> VNFPNIPAEGVRFRLRARDSGYVIYSRTENDPLVWHYNGPPYDDQLFTLIHGTGSRLNLYAIKSVPNGRVLFSRNSASPTVGNIVGDGTYNDNWFQFIQDDNDANSFRIYSLASDSVLYSRTTGAPQFGNYTGPKFDDQLW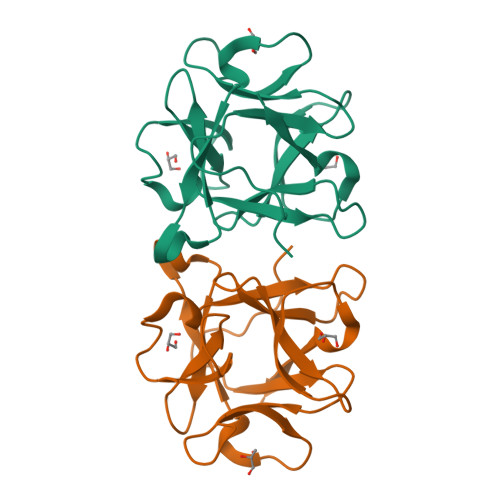HFEIV> MGHLSAPLHRVRVPWQGLLLTASLLTFWNPPTTAQLTTESMPFNVAEGKEVLLLVHNLPQQLFGYSWYKGERVDGNRQIVGYAIGTQQATPGPANSGRETIYPNASLLIQNVTQNDTGFYTLQVIKSDLVNEEATGQFHVYPELPKPSISSNNSNPVEDKDAVAFTCEPETQDTTYLWWINNQSLPVSPRLQLSNGNRTLTLLSVTRNDTGPYECEIQNPVSANRSDPVTLNVTYGPDTPTISPSDTYYRPGANLSLSCYAASNPPAQYSWLINGTFQQSTQELFIPNITVNNSGSYTCHANNSVTGCNRTTVKTIIVTELSPVVAKPQIKASKTTVTGDKDSVNLTCSTNDTGISIRWFFKNQSLPSSERMKLSQGNTTLSINPVKREDAGTYWCEVFNPISKNQSDPIMLNVNYNALPQENGLSPGHHHHHH

The fusobacterial trimeric autotransporter adhesin (TAA) CbpF binds to CEACAM1 on immune cells, resulting in downregulation of their activity against tumors colonized by F. nucleatum. In contrast to Fap2, CbpF is a homotrimeric type Vc autotransporter protein, in which all three protomers together form a trimeric passenger domain that remains exposed on the cell surface after expression, and a C-terminal β-barrel domain that serves as a membrane anchor. The ECD of CEACAM1 comprises an N-terminal, membrane-distal immunoglobulin variable region-like (IgV-like) domain and three membrane-proximal immunoglobulin constant region-like (IgC2-like) domains IgC2-like A1, IgC2-like B, and IgC2-like A2. CbpF binds to CEACAM1 via a protruding loop (D142–Y149) and via H92 on the respective adjacent protomer chain.

Whereas previous structural analysis by X-ray crystallography only resolved the N-terminal IgV-like domain of CEACAM1 (residues 35–142), our cryo-EM structure, after shifting the center of reconstruction toward one CEACAM1, also resolves the following IgC2-like A1 domain (residues 35–234 in total). Although the ECD of CEACAM1 is highly glycosylated and our data revealed several glycosylation sites on the IgV-like and IgC2-like A1 domains, no glycans are involved in the interaction with CbpF. For CEACAM1, the residues with highest SASA differences (F63, Q78, G85, T86, T90, L129) are arranged around a cavity at the tip of the IgV domain where the interaction with CbpF occurs. While the IgC-like domains are heavily glycosylated, the IgV-like domain that is involved in interaction with CbpF is less glycosylated.>MQERIKAC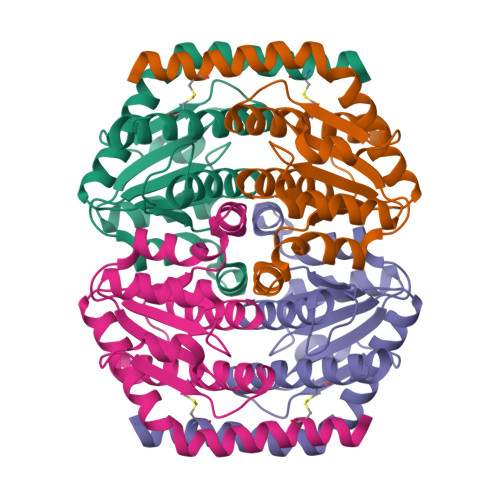FTESIQTQIAAAEALPDAISRAAMTLVQSLLNGNKILCCGNGTSAANAQHFAASMINRFETERPSLPAIALNTDNVVLTAIANDRLHDEVYAKQVRALGHAGDVLLAISTRGNSRDIVKAVEAAVTRDMTIVALTGYDGGELAGLLGPQDVEIRIPSHRSARIQEMHMLTVNCLCDLIDNTLFPHQDD[2x]>[2x]SNAMRVLTGLQPSGDLHIGNYFGAIKQMVDAQEKSQMFMFIANYHAMTSSQDGEKLKQNSLKAAAAFLSLGIDPQKSVFWLQSDVKEVMELYWILSQFTPMGLLERAHSYKDKVAKGLSASHGLFSYPVLMAADILLFDTRIVPVGKDQI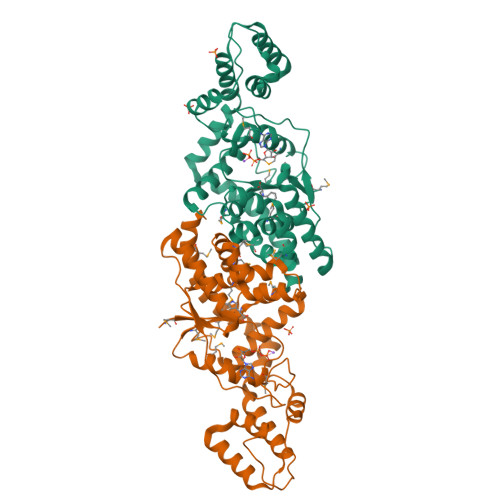QHVEIARDIALKVNNEWGEIFTLPEARVNEEVAVVVGTDGAKMSKSYQNTIDIFSSEKTLKKQISSIVTDSTALEDPKDHENCNIFKIAKLFLDESGQKELQIRYEKGGEGYGHFKIYLNELVNAYFKEAREKYNELLEKPSHLKEILDFGATKARKIAQEKMQKIYEKIGL Propionyl-CoA carboxylase (PCC) and 3-methylcrotonyl-CoA carboxylase (MCC) are biotin-dependent carboxylases (BDCs) that catalyze the metabolism of odd-chain fatty acids, cholesterol, and specific amino acids. In contrast, PCC and MCC have their BC, CT, and BCCP domains divided into two chains: the α subunits contain the BC and BCCP domains, with an intermediate BC-CT interaction (BT) domain between them, while the β subunits solely consist of the CT domain. In humans, PCC and MCC catalyze the carboxylation of propionyl-CoA and 3-methylcrotonyl-CoA (MC-CoA), respectively. (**A, B**) The side view (left) and top view (right) of human PCC holoenzyme (PCC-apo) (**A**) and MCC holoenzyme (MCC-apo) (**B**). Both holoenzymes are dodecamers consisting of six α subunits and six β subunits.

Using the same batch of purified BDCs ([Fig figs1], H to K), we also determined the cryo-EM structures of human PCC and MCC holoenzymes in the acetyl-CoA-bound state (referred to as PCC-ACO and MCC-ACO) at resolutions of 3.38 Å and 2.85 Å, respectively ([Fig figs2], [Fig figs3], I to L, [Fig figs4], I to L, [Fig figs6] and [Fig figs7], [Table tbls1] and [Table tbls2]). The BC domains of one PCCα subunit in the PCC-ACO structure and three MCCα subunits in the MCC-ACO structure are not resolved. These domains were built into the structures based on the resolved BC domains in other α subunits ([Fig figs8], C and F). The PCC-ACO structure closely resembles the PCC-apo and the PCC-PCO structures. The acetyl-CoA in the PCC-ACO structure has a binding mode similar to the propionyl-CoA in the PCC-PCO structure ([Fig fig3]). The conformation of the acyl-CoA binding pocket in both structures is also highly similar ([Fig fig3]). In addition, the well resolved CoA groups of propionyl-CoA and acetyl-CoA bind at the same position in human PCC holoenzyme ([Fig fig3]). These findings indicate that propionyl-CoA and acetyl-CoA bind to PCC with a similar binding mode. Thus, the selectivity of PCC towards propionyl-CoA and acetyl-CoA is largely determined by the interactions between the acyl group and PCC. The longer acyl group in propionyl-CoA, in comparison to that in acetyl-CoA, may mediate a stronger hydrophobic interaction that stabilizes the α carbon of the acyl group at a proper position to react with the carboxylated biotin.

>[6x]MAGFWVGTAPLVAAGRRGRWPPQQLMLSAALRTLKHVLYYSRQCLMVSRNLGSVGYDPNEKTFDKILVANRGEIACRVIRTCKKMGIKTVAIHSDVDASSVHVKMADEAVCVGPAPTSKSYLNMDAIMEAIKKTRAQAVHPGYGFLSENKEFARCLAAEDVVFIGPDTHAIQAMGDKIESKLLAKKAEVNTIPGFDGVVKDAEEAVRIAREIGYPVMIKASAGGGGKGMRIAWDDEETRDGFRLSSQEAASSFGDDRLLIEKFIDNPRHIEIQVLGDKHGNALWLNERECSIQRRNQKVVEEAPSIFLDAETRRAMGEQAVALARAVKYSSAGTVEFLVDSKKNFYFLEMNTRLQVEHPVTECITGLDLVQEMIRVAKGYPLRHKQADIRINGWAVECRVYAEDPYKSFGLPSIGRLSQYQEPLHLPGVRVDSGIQPGSDISIYYDPMISKLITYGSDRTEALKRMADALDNYVIRGVTHNIALLREVIINSRFVKGDISTKFLSDVYPDGFKGHMLTKSEKNQLLAIASSLFVAFQLRAQHFQENSRMPVIKPDIANWELSVKLHDKVHTVVASNNGSVFSVEVDGSKLNVTSTWNLASPLLSVSVDGTQRTVQCLSREAGGNMSIQFLGTVYKVNILTRLAAELNKFMLEKVTEDTSSVLRSPMPGVVVAVSVKPGDAVAEGQEICVIEAMKMQNSMTAGKTGTVKSVHCQAGDTVGEGDLLVELE;>[6x]MAAALRVAAVGARLSVLASGLRAAVRSLCSQATSVNERIENKRRTALLGGGQRRIDAQHKRGKLTARERISLLLDPGSFVESDMFVEHRCADFGMAADKNKFPGDSVVTGRGRINGRLVYVFSQDFTVFGGSLSGAHAQKICKIMDQAITVGAPVIGLNDSGGARIQEGVESLAGYADIFLRNVTASGVIPQISLIMGPCAGGAVYSPALTDFTFMVKDTSYLFITGPDVVKSVTNEDVTQEELGGAKTHTTMSGVAHRAFENDVDALCNLRDFFNYLPLSSQDPAPVRECHDPSDRLVPELDTIVPLESTKAYNMVDIIHSVVDEREFFEIMPNYAKNIIVGFARMNGRTVGIVGNQPKVASGCLDINSSVKGARFVRFCDAFNIPLITFVDVPGFLPGTAQEYGGIIRHGAKLLYAFAEATVPKVTVITRKAYGGAYDVMSSKHLCGDTNYAWPTAEIAVMGAKGAVEIIFKGHENVEAAQAEYIEKFANPFPAAVRGFVDDIIQPSSTRARICCDLDVLASKKVQRPWRKHANIPL The fat mass and obesity associated protein (FTO) is an Fe(II) and 2-oxoglutarate (2OG)-dependent oxygenase that catalyzes the oxidation of N-methyl groups in nucleic acids, and, in particular, of N6-methyladenosine (m6A) in RNA.1−3 FTO is a potential medicinal chemistry target due to its roles in obesity and cancer. Here, we report the use of structural knowledge of how FTO binds 2OG and substrate to design potent and, at least partially selective, FTO inhibitors. Using information from crystal structures of FTO in complex with 2OG and substrate mimics, we designed and synthesized two series of FTO inhibitors, which were characterized by turnover and binding assays, and by X-ray crystallography with FTO and the related bacterial enzyme AlkB. A potent inhibitor employing binding interactions spanning the FTO 2OG and substrate binding sites was identified.

To investigate the generality of the skewed binding mode of 14a as observed with FTO, we solved a crystal structure of a truncated version of the related bacterial NAOX AlkB (AlkBΔN11) in complex with it. By contrast with the crystallographically observed FTO binding mode of 14a, in the AlkB-14a structure, the metal-coordinating atoms of 14a and the metal-ion are co-planar with the pyridinyl ring. Contrary to the binding mode observed with FTO, the p-nitrophenyl group of 14a is directed way from the center of the AlkB active site without significantly displacing key substrate binding side chains. In the case of the structure of the complex of FTOΔ31-14a, a skewed inhibitor binding mode was observed; the skewed binding was less apparent in a structure of the bacterial NAOX AlkBΔN11 in complex with 14a. In contrast, the superimposition of the FTOΔ31-14a and AlkB-14a structures with the PHD2-2 structure reveals that the nitrophenyl group of 14a will likely project into an unoccupied space at the active site entrance of PHD2.

> MLDLFADAEPWQEPLAAGAVILRRFAFNAAEQLIRDINDVASQSPFRQMVTPGGYTMSVAMTNCGHLGWTTHRQGYLYSPIDPQTNKPWPAMPQSFHNLCQRAATAAGYPDFQPDACLINRYAPGAKLSLHQDKDEPDLRAPIVSVSLGLPAIFQFGGLKRNDPLKRLLLEHGDVVVWGGESRLFYHGIQPLKAGFHPLTIDCRYNLTFRQAGKKE>HHHHHHNKDLKGLYAALLVPFDENGQVNEQGLKQIAQNAIETEELDGLYVNGSSGENFLLNTEQKKQVFKVAKEAVGDKVKLIAQVGSLDLNEAIELGKYATELGYDALSAVTPFYYPFTFEEIRDYYFDIIEATQNNMIIYAIPDLTGVNISIEQFSELFNHEKIVGVKYTAPNFFLLERIRKAFPDKLILSGFDEMLVQATISGVDGAIGSTYNVNGRRARKIFDLARQGQIQEAYQLQHDSNDIIETVLSMGIY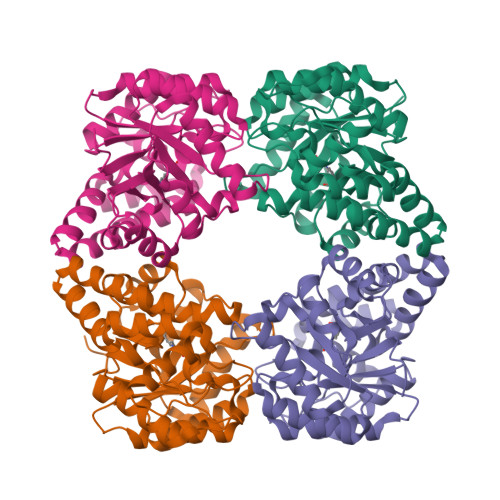PTLKEILRHRGIDAGLPKRPFKPFNEAHRQTLDQLIAKYDL[4x]Histidine phosphotransfer (HPt) proteins allow bacteria, yeast, and plants to expand beyond canonical two-component signaling pathways into multi-step phosphorelay pathways. The pathway consists of the transmembrane HHK Sln1, the HPt Ypd1, and the RR proteins Ssk1 and Skn7. The HPt protein (or domain) acts as an intermediate in the signaling pathway by transferring the phosphoryl group from the HHK to a RR, which elicits a cellular response to the detected stress. All known structures of HPt proteins share a characteristic 4-helix bundle with a hydrophobic binding surface for RR binding.

The X-ray structure of the Ypd1-G68Q mutant was determined in order to ascertain structural integrity of the mutant and to gain insight into its loss of function characteristics. The Ypd1-G68Q mutant protein crystallized in space group P3121. The structure was solved to a resolution of 1.98 Å using molecular replacement. Clear electron density was observed for the side chain of the glutamine substitution at position 68. The root mean square deviation (RMSD) for all residues between the Ypd1-G68Q and wild type structure is 1.9 Å. The area around the site of phosphorylation is unperturbed with an RMSD of 0.2 Å for all residues in αC and αD helix. The N-terminal αA helix and the following turn (residues 11–21) show the largest shifts in the C-alpha positions with an RMSD of 1.7 Å. The αB helix is extended by one turn (residues 22–26) in the Ypd1-G68Q structure. The αA helix rotates approximately 30° around an axis at its N-terminus and αA helix makes a ¼ rotation around its longitudinal axis. Upon the αA twisting movement, the originally exposed I13 and I17 become buried, while L14 and I18 are now exposed.

> MSTIPSEIINWTILNEIISMDDDDSDFSKGLIIQFIDQAQTTFAQMQRQLDGEKNLTELDNLGHFLKQSSAALGLQRIAWVCERIQNLGRKMEHFFPNKTELVNTLSDKSIINGINIDEDDEEIKIQVDDKDENSIYLILIAKALNQSRLEFKLARIELSKYYNTNL PepP encodes an enzyme belonging to the aminopeptidases P (APPro) family (E.C.3.4.11.9), a type of metalloprotease that catalyzes the removal of the N-terminal residue from a polypeptide that has proline as the second residue. It is one of the critical virulence-associated genes identified using a P. aeruginosa-C. elegans infection mode. In contrast to other metalloaminopeptidases, APPro is a cytoplasmic aminopeptidase and recognizes a restricted scissile Xaa-Pro bond of those polypeptide or protein substrates that may be linked to virulence-associated phenotypes or other biological processes beyond the general protein degradation ability. In this study, we solved the X-ray crystal structure of Pa-PepP with a resolution of 1.8 Å.

The monomer structure displays a two-domain organization where the N-domain (1–175) is composed of a mainly parallel beta-sheet core (B1–B6) flanked by seven alpha helices (A–G). In contrast, the catalytic C- domain (176–444) adopts a conserved “pita-bread” fold with six beta sheets (B7-B12) in antiparallel configurations. The monomers were arranged as a dimer with an extended loop contributing to the active site of the adjacent subunit and an average interface area of approximately 2050.9 A2 per subunit. To identify the binding state of Mn2+ ions in active site, 10 mM MnCl2 was added during the crystallization experiment, along with 10 mM proline. In the final structure, there are three Mn atoms in each monomer. MnA is liganded by the side chains of His354, Asp271, Glu384, Glu408, and MnB interacts with Asp260, Asp271, Glu408. The smaller anomalous signals and 0.5 occupancies of the MnB site confirmed one of the structural features in metal-dependent aminopeptidase: the metal binding site B has relatively weaker binding affinity comparing to the site A. Additionally, the third Mn atom (MnC) is located in a position previously identified as being occupied by water in Zn-load Ec-PepP structures. In Pa-PepP, MnC interacts through one solvent molecular (W) with MnA and MnB, with a metal-separation distance of 3.1–3.7 Å. Remarkably, MnC occupies the S1 subsite that ordinarily binds the substrate, providing an explanation for the inhibition effect of excessive metal binding. The modeled tripeptide-bound Pa-PepP structure indicated that Arg153 and Arg351 accommodate the carboxylate group of the P2’ Leu, and guide the C-terminus of the substrate toward the tetramer surface.

>MIRIPKSEYARRRKALMAQMEPNSIAILPAAPMYIRNRDVEHVYRQDSDFQYLTGFPEPEAVMALIPGRAHGEYVLFCRERDPERELWDGLRAGQDGAIGQYGADDAFPIGDIDDILPGLIEGRDRVYYALGANPDFDRRLMDWINVIRSKARQGAQPPNEFVALDHLLHDQRLYKSANEVKVMRYAAEVSARAHIRAMEVCRPGLFEYHLEAELEYEFRKGGAKMPAYGSIVAAGRNACILHYRENDAAIKDGDLILIDAGCEIDCYASDITRTFPANGRFSPEQKAIYELVLEANMAAFDYIAPGRHWNEAHEATVRVITAGLVRLGLLEGDVDELIAHEAYKAFYMHRAGHWLGMDVHDVGEYRVGGEWRVLEPGMAMTVEPGIYIAPDNTTVAKKWRGIGVRIEDDVVVTRNGCEVLTNGVPKTVAEIEALMAAAKSEAALEHHHHHH[4x]> MGSSHHHHHHSQDPSEIWRQCKGERHIRPLQGRLVRLVESQDQVATLQLVDTLEEQALLEELLESSKPPVPADAEPLHYLLKTPFRYPPLRWGSRFGRRHEPSL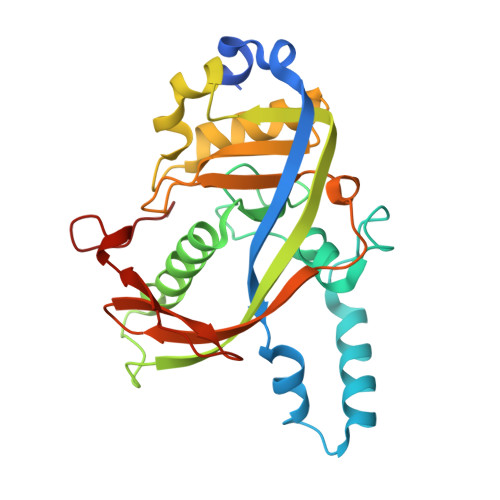FYAALKLETAMAESAYYRCVLWSGMVVPPPSGRILSEHASFEAGWKVERGIRLQAPPFSDHEAALTDIADYRAPQELGSAMRSAGVQAFEYRSARCPERGCNVALFTPAAFTEKRPRNLTPWLCETTAGYVAFKPAHVPGSPKIFSWELFLVDGKLPHPA> GSMASAPLRVYVQCNPLLDVSAHVSDEFLVKYGLERGTAILLSERQKGIFDDIEKMPNVRYVPGGSGLNVARVAQWMQQAYKGKFVTYVGCIADDRYGKVLKEAAEHEGIVMAVEHTTKAGSGACAVCITGKERTLVADLGAANHLSSEHMRSPAVVRAMDESRIFYFSGFTLTVDVNHVLQACRKAREVDGLFMINLSAPFIMQFFSAQLGEVLPYTDIIVANRHEAKEFANMMKWDTDCVEEIARRAVSEVPYTGTKGRVVVFTRDIESTVLATKDGVETVPVPQLDQDKVIDMNGAGDAFMGGFLSAYA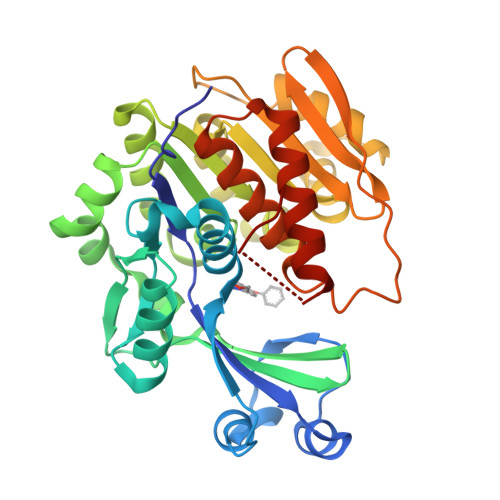VGKDLRRCCETGHYTAQEVIQRDGCSFPEKPSFSP>[4x]EKDKIKFLLVEGVHQKALESLRAAGYTNIEFHKGALDDEQLKESIRDAHFIGLRSRTHLTEDVINAAEKLVAIGAFAIGTNQVDLDAAAKRGIPVFNAPFSNTRSVAELVIGELLLLLRGVPEANAKAHRGVGNKLAAGSFEARGKKLGIIGYGHIGTQLGILAES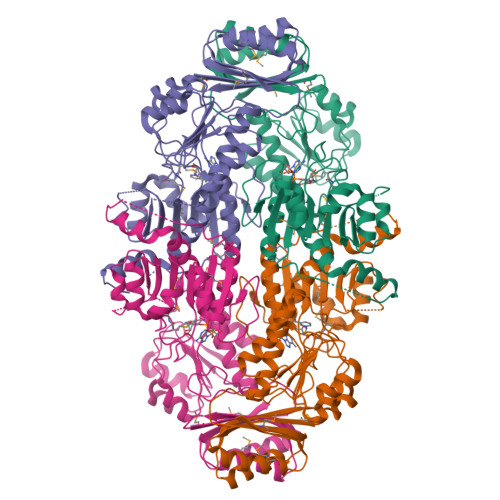LGMYVYFYDIENKLPLGNATQVQHLSDLLNMSDVVSLHVPENPSTKNMMGAKEISLMKPGSLLINASRGTVVDIPALADALASKHLAGAAIDVFPTEPATNSDPFTSPLAEFDNVLLTPHIGGSTQEAQENIGLEVAGKLIKYSDNGSTLSAVNFPEVSLPLHGGRRLMHIHENRPGVLTALNKIFAEQGVNIAAQYLQTSAQMGYVVIDIEADEDVAEKALQAMKAIPGTIRARLLY>[17x]SIYPKFRAAAVQAAPIYLNLEASVEKSCELIDEAASNGAKLVAFPEAFLPGY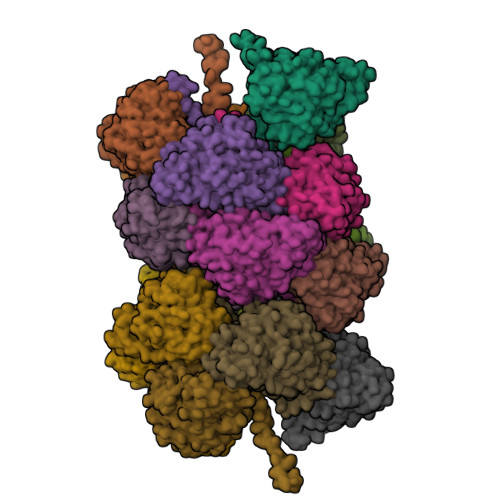PWFAFIGHPEYTRKFYHELYKNAVEIPSLAIQKISEAAKRNETYVCISCSEKDGGSLYLAQLWFNPNGDLIGKHRKMRASVAERLIWGDGSGSMMPVFQTEIGNLGGLMCWEHQVPLDLMAMNAQNEQVHVASWPGYFDDEISSRYYAIATQTFVLMTSSIYTEEMKEMICLTQEQRDYFETFKSGHTCIYGPDGEPISDMVPAETEGIAYAEIDVERVIDYKYYIDPAGHYSNQSLSMNFNQQPTPVVKHLNHQKNEVFTYEDI We showed by HPAEC-PAD and LC-FD-MS/MS that RgGH98 is specific for blood group A tetrasaccharide type II (BgA II). As expected from the construct, RgGH98 adopts a modular structure with 3 domains. Structural alignment to homologous GH98 enzymes identified the binding pocket and the general acid catalytic residue as Glu 411, which is present in a cleft in the centre of the Cd. Fragmentation of this species showed that the deoxy-hexose was linked to the hexose at the reducing end, as determined by the characteristic fragments at 431 and 449 Da. Together, the HPAEC-PAD and MS/MS analyses confirmed that BgAtri was released from mucin following RgGH98 hydrolysis of the Galβ1-4GlcNAc glycosidic linkage in BgA II.

The N-term domain identified as GBLD, residues 55 to 260, presents a β-sandwich fold. Two loops, comprising residues 79 to 105 and 138 to 163, extend from the GBLD and wrap around the Cd. The C-term domain, residues 592 to 876 aa, with a central β-sandwich module follows. Additional calcium and magnesium ions were modelled in the RgGH98–BgAtri complex and RgGH98 apo crystal structures. However, in these experiments both ions were present at a concentration of 50 mM, increasing the likelihood of nonspecific binding.

>KAPPLVNLAEEKDVKVTVGENMDLKNADLLTDGDKYYLQHDATGNKEGNNWENYQEQGTEVTSTAEGKNGVWVQVDLGASYPLEVINLKRQVYDGQATIGNGNPSGQGKRLKGTKISYKNTAIVIGNEEDLSDGQIVYYEGNPTLPDGVKQPENVSKPYEEAMGGQWFYMDYANKNGLGATELGTTKEARYIRVYTENPKGAAVKFMELGIYGYENEQDVQSQDGPRRVIDNEHPMMIATAYSNDVYEIGQEEGPELQGSNTVDGRWNAIPDDLKENNVLLLHTNNLRQFAPDHIGQAYLQAFHEHGLQIAYEQGAPIMLLGLTAAATPENGGTQYNITADMDYGWLDLMYRMYPNMQGVFNTENFWAGIHPPCEGSAKMLEIADRFGGFFVWSDQDHGSTVTNIVSNANMKKALEKHGDAFYLIYKNTSSNQPDDLKTSSFFQGSWLAGYTGGWGMLSDTWAWDKQFSKLWQGAGSYNNWQRLCGEPEALLGMQMMSTYLGGGVIYTFEFPEIVYGTSNTNSPANTHVLTELFRYIVNHPAPSKKEIMEETKAVLYGNVSSDFYSGLSGKPTGFQIYETGRYGIIPVIPTWGTRAEVTKKLIQEADKLGVTPPNVLDVKDKNLSGQAKQKYFKDLYPIEYVGNAFADKWEGTWYLYNNKVNTNEKQHAILPLEGEEESARLKVEMEPHEFMIMNESGDGTAMDITLNNYRVNKDEIIFDNKFGLTWTGDFSPGQTTINGKLSVYKYMDEYNVVNAPEGKLSPEDNELRTTTFELTKLAKEPKVQVVKGQQPDTDGQPQYTEPKVEFNEETGKAVITIQTNGWVDLSITGLEFVYDENAQKIEDEPIKS[2x]> 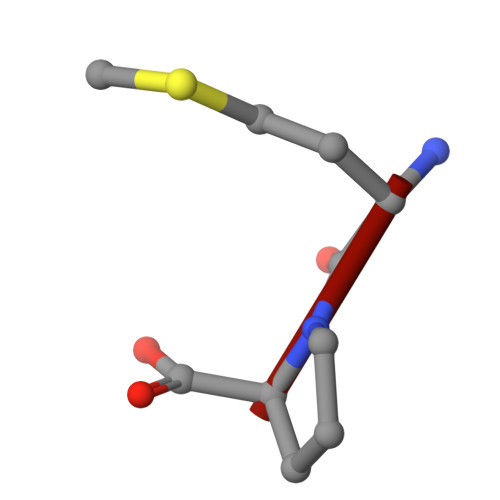MP> MSMLKREDWYDLTRTTNWTPKYVTENELFPEEMSGARGISMEAWEKYDEPYKITYPEYVSIQREKDSGAYSIKAALERDGFVDRADPGWVSTMQLHFGAWALEEYAASTAEARMARFAKAPGNRNMATFGMMDENRHGQIQLYFPYANVKRSRKWDWAHKAIHTNEWAAIAARSFFDDMMMTRDSVAVSIMLTFAFETGFSNMQFLGLAADAAEAGDHTFASLISSIQTDESRHAQQGGPSLKILVENGKKDEAQQMVDVAIWRSWKLFSVLTGPIMDYYTPLESRNQSFKEFMLEWIVAQFERQLLDLGLDKPWYWDQFMQDLDETHHGMHLGVWYWRPTVWWDPAAGVSPEEREWLEEKYPGWNDTWGQCWDVITDNLVNGKPELTVPETLPTICNMCNLPIAHTPGNKWNVKDYQLEYEGRLYHFGSEADRWCFQIDPERYKNHTNLVDRFLKGEIQPADLAGALMYMSLEPGVMGDDAHDYEWVKAYQKKTNAA;> MSEQQPEALKPLKTWSHLAGNRRRPSEYEVVSTNLHYFTDNPERPWELDSNLPMQTWYKKYCFDSP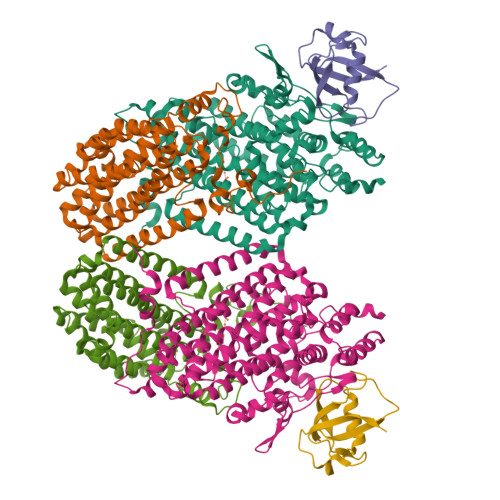LKHDDWNAFRDPDQLVYRTYNLLQDGQESYVQGLFDQLNDRGHDQMLTREWVETLARFYTPARYLFHALQMGSVYIHQIAPASTITNCATYETADHLRWLTHTAYRTRELANCYPDVGFGKRERDVWENDPAWQGFRELIEKALIAWDWGEAFTAINLVTKPAVEEALLQQLGSLAQSEGDTLLGLLAQAQKRDAERHRRWSSALVKMALEKEGNREVLQKWVAKWEPLADKAIEAYCSALPDGENAIVEAKSASRYVRQMMGL;> MATFPIMSNFERDFVIQLVPVDTEDTMDQVAEKCAYHSINRRVHPQPEKILRVRRHEDGTLFPRGMIVSDAGLRPTETLDIIFMDN>STPGAQEVLFRTGIAAVNSTNHLRVYFQDSHGSIRESLYESGWANGTAKNVIAKAKLGTPLAATSKELKNIRVYSLTEDNVLQEAAYDSGSGWYNGALAGAKFTVAPYSRIGSVFLAGTNALQLRIYAQKTDNTIQEYMWNGDGWKEGTNLGVALPGTGIGVTCWRYTDYDGPSIRVWFQTDNLKLVQRAYDPHTGWYKELTTIFDKAPPRCAIAATNFNPGKSSIYMRIYFVNSDNTIWQVCWDHGQGYHDKRTITPV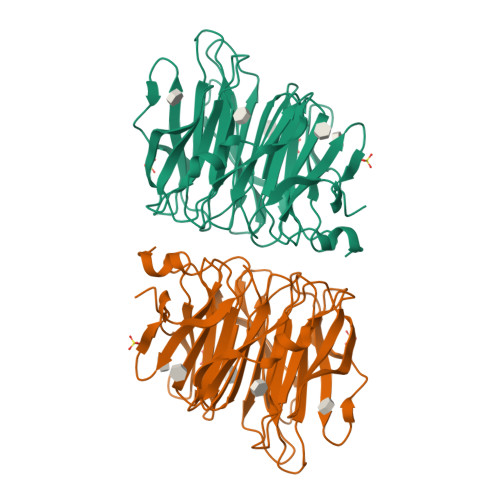IQGSEIAIISWEGPELRLYFQNGTYVSAISEWTWGKAHGSQLGRRALPPAE[3x]>SNAMKIKKESLEMRQMRKKVVLIGTGLIGGSLALAIKKDHDVTITGYDIFQEQVERAKELHVVDEIAVDLQHACEEAHLIVFASPVEETKKLLHKLASFHLREDVIVTDVGSTKGSIMNEAEALFSKEISFIGGHPMAGSHKTGVESAKAHLFENAFYILTPMHHVPNEHVEELKDWLKGTGSHFLVLNTEEHDYVTGIVSHFPHLIAAGLVKQVEKHAGDNPLIHQLAAGGFKDITRIASSSPKMWSDIVKQNREHLMVLLKEWISEMEDLYDTVSSGDAGE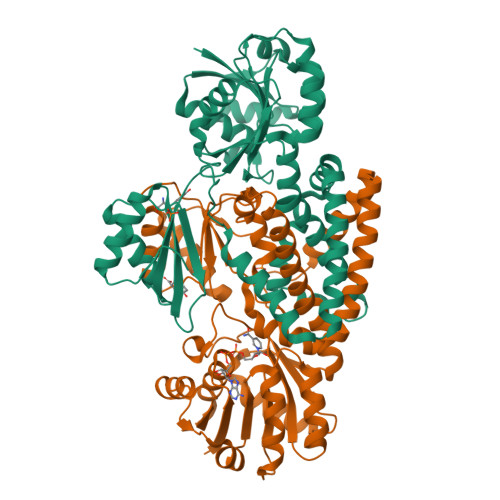IQNYFADAKEYRDSLPVRKRGAIPAYHDLYVDVLDKVGALAHVTSILAREEISITNLQILEAREGLLGVLRISFQREEDRMKAKLALGEEKYQTYETI[2x]>[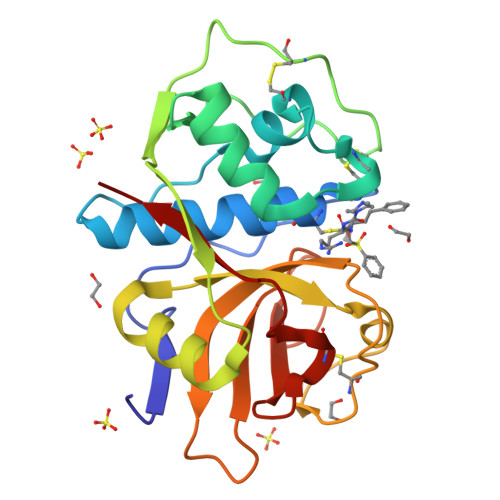2x]APAAVDWRARGAVTAVKDQGQCGSCWAFSAIGNVECQWFLAGHPLTNLSEQMLVSCDKTDSGCSGGLMNNAFEWIVQENNGAVYTEDSYPYASGEGISPPCTTSGHTVGATITGHVELPQDEAQIAAWLAVNGPVAVAVDASSWMTYTGGVMTSCVSEQLDHGVLLVGYNDSAAVPYWIIKNSWTTQWGEEGYIRIAKGSNQCLVKEEASSAVVG> MSQSKKETPLASLLFDDVEKINHDQDYWFQLRGDNPNVLIDAATPLFGLSLRVRTLTECDNIEQIYRQTIEEIKAIEIELTEQGYEHAILMAYRYILCAFLDESVMGTEWGA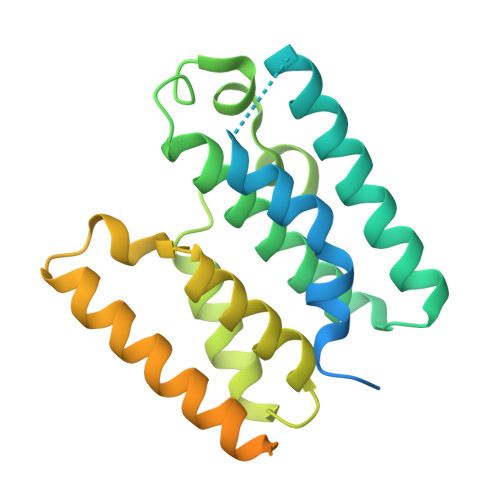SSLWAEHSMLSRFHNETWGGEKVFTILSRLEGEPHRYQALLAFIYHCLILGFEGKYRVMEGGQAEREKVISRLHQLLSSLEESEPQDLTRPTDHVVRAKYTLSRQMPVWSVFAGFIVLWVGLFLGYSYVLHSKSSDVLNQLNQIL> MVAGHASGSPAFGTASHSNCEHEEIHLAGSIQPHGALLVVSEHDHRVIQASANAAEFLNLGSVLGVPLAEIDGDLLIKILPHLDPTAEGMPVAVRCRIGNPSTEYCGLMHRPPEGGLIIELERAGPSIDLSGTLAPALERIRTAGSLRALCDDTVLLFQQCTGYDRVMVYRFDEQGHGLVFSECHV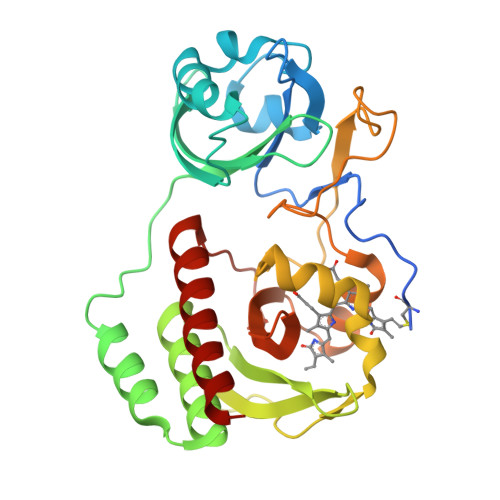PGLESYFGNRYPSSLVPQMARQLYVRQRVRVLVDVTYQPVPLEPRLSPLTGRDLDMSGCFLRSMSPIHLQFLKDMGVRATLAVSLVVGGKLWGLVVCHHYLPRFIRFELRAICKRLAERIATRITALES>MKIRIGHGFDVHKFGEPRPLILCGVEVPYETGLVAHSDGDVVLHAISDAILGAMALGDIGKHFPDTDAAYKGADSRVLLRHCYALAKAKGFELGNLDVTIIAQAPKMAPHIEDMRQVLAADLNADVADINVKATTTEKLGFTGRKEGIAVEAVVLL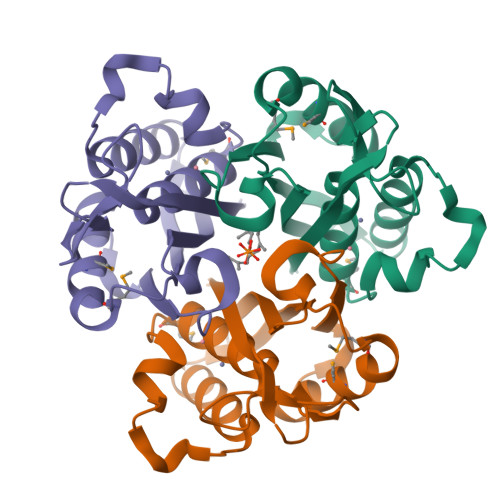SRQ[3x]Mitochondrial calcium uptake is mediated by the mitochondrial calcium uniporter, a Ca2+-selective channel that is localized to the inner mitochondrial membrane. In humans, the uniporter functions as a holocomplex (referred to as uniplex henceforth) and consists of the pore-forming subunit MCU, an essential membrane-spanning subunit EMRE, and the gate-keeping subunits MICU1 and MICU2. The two-transmembrane (2-TM) MCU component forms a tetrameric channel pore and the single-TM EMRE becomes an integral part of the channel by forming a 1:1 stoichiometric subcomplex with MCU and renders the channel conductive. MICU1 and MICU2 are two paralogous EF-hand containing proteins that are localized to the mitochondrial intermembrane space (IMS) and function as gate-keepers by sensing the cytosolic Ca2+ concentration and, thereby, regulate MCU-EMRE channel activity.

The major class of particles (class 1) represents a blocked uniplex in which a heterodimer of MICU1 and MICU2 blocks the central ion conduction pore of a monomeric MCU-EMRE subcomplex. Similar MICU1-MICU2 blocking is also observed in the second class (class 2) with the exception being that MCU-EMRE subcomplex retains its dimeric form. By C2 symmetry expansion, particles of this class were combined with those of class one and yielded the structure of a blocked uniplex at 4.6 Å resolution (Figure 1—figure supplements 4 and 5, and Figure 1—source data 1). In the blocked uniplex structure, MICU1 engages with the MCU-EMRE subcomplex at three major points of contact using its N- and C-terminal helices. Firstly, the α1 helix of MICU1 is oriented directly above the ion conduction pore with its N-terminus pointing toward the C-terminus of the EMRE helix. This would position the N-terminal poly-basic region of MICU1 within the proximity of the C-terminal poly-aspartate tail of EMRE, allowing for the formation of a putative salt-bridge network. Secondly, the α2 helix is positioned directly above the D-ring of MCU’s selectivity filter, which is formed by the four Asp261s from the DIME motif at the external entrance of the channel tetramer. Several basic residues from MICU1 are in close proximity and can potentially engage in electrostatic interactions with the MCU D-ring Asp261s, including K126 and R129 in α2 as well as the basic resides (R259, R261 and R263) in the loop between α7 and α8, which is disordered in the Ca2+-bound MICU1. Most notably, Lys126 is well positioned to point its side chain directly toward the center of the D-ring and block the channel filter. Thirdly, the amphipathic C-terminal helix (C-helix, α17) of MICU1 lies on the membrane surface between two neighboring EMRE subunits with its N-terminus sandwiched between the C-termini of an EMRE helix and the TM1 from a neighboring MCU subunit. In the absence of Ca2+, MICU1 from the MICU1-MICU2 dimer engages in more extensive interactions with both EMRE and the MCU pore of the MCU-EMRE subcomplex, blocking the channel’s external entrance.

>[4x]MAAAAGRSLLLLLSSRGGGGGGAGGCGALTAGCFPGLGVSRHRQQQHHRTVHQRIASWQNLGAVYCSTVVPSDDVTVVYQNGLPVISVRLPSRRERCQFTLKPISDSVGVFLRQLQEEDRGIDRVAIYSPDGVRVAASTGIDLLLLDDFKLVINDLTYHVRPPKRDLLSHENAATLNDVKTLVQQLYTTLCIEQHQLNKERELIERLEDLKEQLAPLEKVRIEISRKAEKRTTLVLWGGLAYMATQFGILARLTWWEYSWDIMEPVTYFITYGSAMAMYAYFVMTRQEYVYPEARDRQYLLFFHKGAKKSRFDLEKYNQLKDAIAQAEMDLKRLRDPLQVHLPLRQIGEKD;>[4x]MASGAARWLVLAPVRSGALRSGPSLRKDGDVSAAWSGSGRSLVPSRSVIVTRSGAILPKPVKMSFGLLRVFSIVIPFLYVGTLISKNFAALLEEHDIFVPEDDDDDD;> MFRLNSLSALAELAVGSRWYHGGSQPIQIRRRLMMVAFLGASAVTASTGLLWKRAHAESPPCVDNLKSDIGDKGKNKDEGDVCNHEKKTADLAPHPEEKKKKRSGFRDRKVMEYENRIRAYSTPDKIFRYFATLKVISEPGEAEVFMTPEDFVRSITPNEKQPEHLGLDQYIIKRFDGKKISQEREKFADEGSIFYTLGECGLISFSDYIFLTTVLSTPQRNFEIAFKMFDLNGDGEVDMEEFEQVQSIIRSQTSMGMRHRDRPTTGNTLKSGLCSALTTYFFGADLKGKLTIKNFLEFQRKLQHDVLKLEFERHDPVDGRITERQFGGMLLAYSGVQSKKLTAMQRQLKKHFKEGKGLTFQEVENFFTFLKNINDVDTALSFYHMAGASLDKVTMQQVARTVAKVELSDHVCDVVFALFDCDGNGELSNKEFVSIMKQRLMRGLEKPKDMGFTRLMQAMWKCAQETAWDFALPKQ;> MAAAAGSCARVAAWGGKLRRGLAVSRQAVRSPGPLAAAVAGAALAGAGAAWHHSRVSVAARDGSFTVSAQKNVEHGIIYIGKPSLRKQRFMQFSSLEHEGEYYMTPRDFLFSVMFEQMERKTSVKKLTKKDIEDTLSGIQTAGCGSTFFRDLGDKGLISYTEYLFLLTILTKPHSGFHVAFKMLDTDGNEMIEKREFFKLQKIISKQDDLMTVKTNETGYQEAIVKEPEINTTLQMRFFGKRGQRKLHYKEFRRFMENLQTEIQEMEFLQFSKGLSFMRKEDFAEWLLFFTNTENKDIYWKNVREKLSAGESISLDEFKSFCHFTTHLEDFAIAMQMFSLAHRPVRLAEFKRAVKVATGQELSNNILDTVFKIFDLDGDECLSHEEFLGVLKNRMHRGLWVPQHQSIQEYWKCVKKESIKGVKEVWKQAGKGLF> MSHTIERPSRLDTARRAFSWRDAVVYQVYLRSFRDANGDGIGDLGGLSQGLDAIAALGCDAIWLNPCYASPQRDHGYDIADYLTIDPAYGTLEEFDEVVRRAHELGLRVLMDMVANHCSSDHAWFQAALAAEPGSDERARFIFRDGLGPDGELPPNNWDSVFGGLAWTRVTERDGRPGQWYLHSFDTSQPDFDWRHPAVAEHFENVLRFWFERGVDGFRIDVAHGHFKDAALPDHPGGRGPDAGHNHGMWDQPEVHDLYRSWRALGDAYEPEKYFVGEIWVPSPDRLADYLRPDELHNAFSFDLLVQPWNADRFRKAIETGLAVGRGWPAWTLANHDVHRAVTRYGQEQPLDEALPTDMIAAARR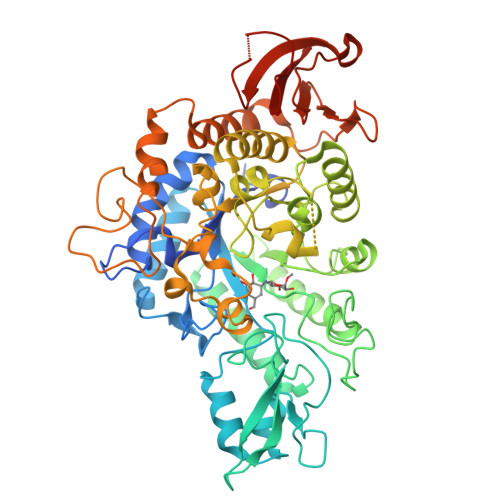RGPADLDRGLRRARAAAALALALPGSMYLYQGEELGLPEVLDLPDAARQDPIWTRSNGTELGRDGCRIPLPWTREGRTFGFSDAAAATTWLPQPAWFGAFARATQAADPDSMLSLHRDLLATRRTHLRGTEPIVWLSPAGAEVLAFRRGDVVVVTNFGSAPFTPPSAWGALSPLLASQPLTGSATVPPETTVWSRLHRGVAALEHHHHHH>[2x]VKSKAKKTVDKHSDEYKIRRERNNIAVRKSRDKAKMRNLETQHKVLELTAENERLQKKVEQLSRELSTLRNLFKQLPE;> GELVRTDSPNFLCSVLPTHWRCNKTLPIAFKVVALGDVPDGTLVTVMAGNDENYSAELRNATAAMKNQVARFNDLRFVGRSGRGKSFTLTITVFTNPPQVATYHRAIKITVDGPREPRRHRQK;> MPRVVPDQRSKFENEEFFRKLSRECEIKYTGFRDRPHE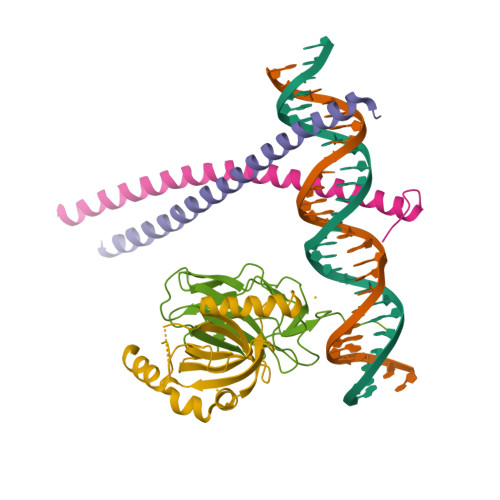ERQTRFQNACRDGRSEIAFVATGTNLSLQFFPASWQGEQRQTPSREYVDLEREAGKVYLKAPMILNGVCVIWKGWIDLHRLDGMGCLEFDEERAQQEDALAQQ> KQTARXSTGG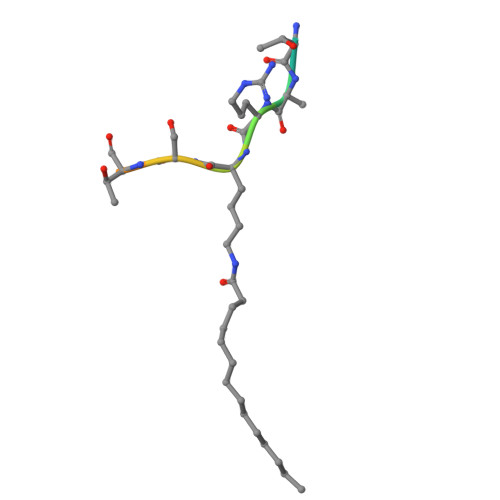WW>[4x]MTMMTATQALSVNPATGQTLAAMPWANAQEIEHALSLAASGFKKWKMTSVA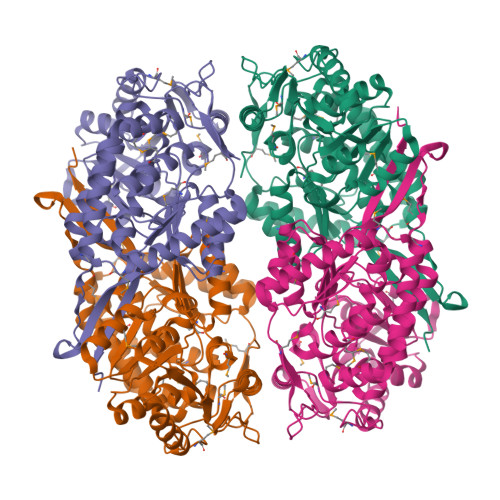QRAQTLRDIGQALRAHAEEMAQCITREMGKPIKQARAEVTKSAALCDWYAEHGPAMLNPEPTLVENQQAVIEYRPLGVILAIMPWNFPLWQVLRGAVPILLAGNSYLLKHAPNVTGCAQMIARILAEAGTPAGVYGWVNANNEGVSQMINDPRIAAVTVTGSVRAGAAIGAQAGAALKKCVLELGGSDPFIVLNDADLELAVKAAVAGRYQNTGQVCAAAKRFIVEEGIAQAFTDRFVAAAAALKMGDPLVEENDLGPMARFDLRDELHQQVQASVAEGARLLLGGEKIAGEGNYYAATVLADVTPDMTAFRQELFGPVAAITVAKDAAHALALANDSEFGLSATIFTADDTLAAEMAARLECGGVFINGYSASDARVAFGGVKKSGFGRELSHFGLHEFCNVQTVWKNRV[(2S)-2-[(2S)-butan-2-yl]-4-(5-chloro-1,3-benzoxazol-2-yl)-1,4-diazepan-1-yl][5-methyl-2-(2H-1,2,3-triazol-2-yl)phenyl]methanone 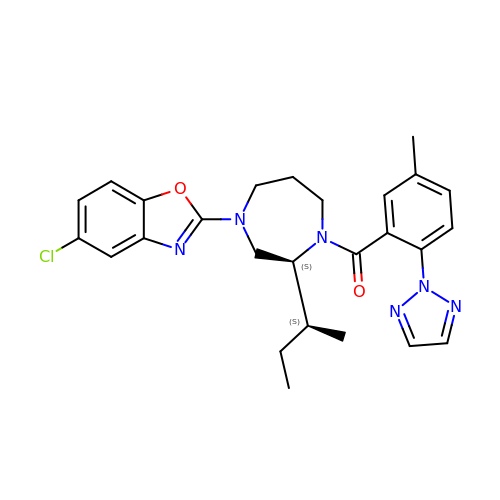| C26 H29 Cl N6 O2 | CRLKYMWQHWKXAE-FDDCHVKYSA-N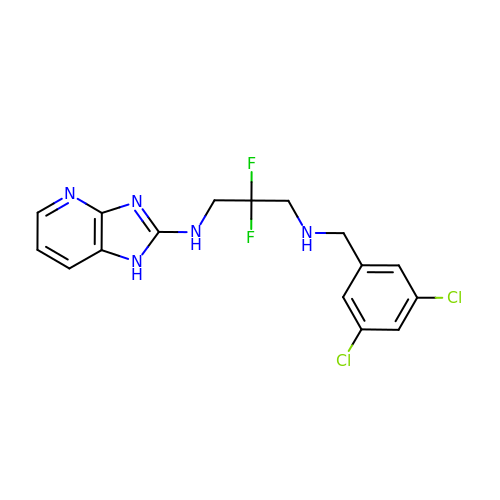N-(3,5-dichlorobenzyl)-2,2-difluoro-N'-(1H-imidazo[4,5-b]pyridin-2-yl)propane-1,3-diamine | C16 H15 Cl2 F2 N5 | MEIIHMGWEAIZIU-UHFFFAOYSA-N>MAEYKDNLLGEANSFLEVLEQVSHLAPLDKPVLIIGERGTGKELIASRLHYLSSRWQGPFISLNCAALNENLLDSELFGHEAGAFTGAQKRHPGRFERADGGTLFLDELATAPMMVQEKLLRVIEYGELERVGGSQPLQVNVRLVCATNADLPAMVNEGTFRADLLDRLAFDVVQLPPLRERESDIMLMAEYFAIQMCREIKLPLFPGFTERARETLLNYRWPGNIRELKNVVERSVYRHGTSDYPLDDIIIDPFKRRP[6x];>MQGSVTEFLKPRLVDIEQVSSTHAKVTLEPLERGFGHTLGNALRRILLSSMPGCAVTEVEIDGVLHEYSTKEGVQEDILEILLNLKGLAVRVQGKDEVILTLNKSGIGPVTAADITHDGDVEIVKPQHVICHLTDENASISMRIKVQRGRGYVPASTRIHSEEDERPIGRLLVDACYSPVERIAYNVEAARVEQRTDLDKLVIEMETNGTIDPEEAIRRAATILAEQLEAFVDLRDVRQPEVKEEKPEFDPILLRPVDDLELTVRSANCLKAEAIHYIGDLVQRTEVELLKTPNLGKKSLTEIKDVLASRGLSLGMRLENWPPASIADE[2x];> MVYSYTEKKRIRKDFGKRPQVLDVPYLLSIQLDSFQKFIEQDPEGQYGLEAAFRSVFPIQSYSGNSELQYVSYRLGEPVFDVQECQIRGVTYSAPLRVKLRLVIYEREAPEGTVKDIKEQEVYMGEIPLMTDNGTFVINGTERVIVSQLHRSPGVFFDSDKGKTHSSGKVLYNARIIPYRGSWLDFEFDPKDNLFVRIDRRRKLPATIILRALNYTTEQILDLFFEKVIFEIRDNKLQMELVPERLRGETASFDIEANGKVYVEKGRRITARHIRQLEKDDVKLIEVPVEYIAGKVVAKDYIDESTGELICAANMELSLDLLAKLSQSGHKRIETLFTNDLDHGPYISETLRVDPTNDRLSALVEIYRMMRPGEPPTREAAESLFENLFFSEDRYDLSAVGRMKFNRSLLREEIEGSGILSKDDIIDVMKKLIDIRNGKGEVDDIDHLGNRRIRSVGEMAENQFRVGLVRVERAVKERLSLGDLDTLMPQDMINAKPISAAVKEFFGSSQLSQFMDQNNPLSEITHKRRISALGPGGLTRERAGFEVRDVHPTHYGRVCPIETPEGPNIGLINSLSVYAQTNEYGFLETPYRKVTDGVVTDEIHYLSAIEEGNYVIAQANSNLDEEGHFVEDLVTCRSKGESSLFSRDQVDYMDVSTQQVVSVGASLIPFLEHDDANRALMGANMQRQAVPTLRADKPLVGTGMERAVAVDSGVTAVAKRGGVVQYVDASRIVIKVNEDEMYPGEAGIDIYNLTKYTRSNQNTCINQMPCVSLGEPVERGDVLADGPSTDLGELALGQNMRVAFMPWNGYNFEDSILVSERVVQEDRFTTIHIQELACVSRDTKLGPEEITADIPNVGEAALSKLDESGIVYIGAEVTGGDILVGKVTPKGETQLTPEEKLLRAIFGEKASDVKDSSLRVPNGVSGTVIDVQVFTRDGVEKDKRALEIEEMQLKQAKKDLSEELQILEAGLFSRIRAVLVAGGVEAEKLDKLPRDRWLELGLTDEEKQNQLEQLAEQYDELKHEFEKKLEAKRRKITQGDDLAPGVLKIVKVYLAVKRRIQPGDKMAGRHGNKGVISKINPIEDMPYDENGTPVDIVLNPLGVPSRMNIGQILETHLGMAAKGIGDKINAMLKQQQEVAKLREFIQRAYDLGADVRQKVDLSTFSDEEVMRLAENLRKGMPIATPVFDGAKEAEIKELLKLGDLPTSGQIRLYDGRTGEQFERPVTVGYMYMLKLNHLVDDKMHARSTGSYSLVTQQPLGGKAQFGGQRFGEMEVWALEAYGAAYTLQEMLTVKSDDVNGRTKMYKNIVDGNHQMEPGMPESFNVLLKEIRSLGINIELED;> MKDLLKFLKAQTKTEEFDAIKIALASPDMIRSWSFGEVKKPETINYRTFKPERDGLFCARIFGPVKDYECLCGKYKRLKHRGVICEKCGVEVTQTKVRRERMGHIELASPTAHIWFLKSLPSRIGLLLDMPLRDIERVLYFESYVVIEGGMTNLERQQILTEEQYLDALEEFGDEFDAKMGAEAIQALLKSMDLEQECEQLREELNETNSETKRKKLTKRIKLLEAFVQSGNKPEWMILTVLPVLPPDLRPLVPLDGGRFATSDLNDLYRRVINRNNRLKRLLDLAAPDIIVRNEKRMLQEAVDALLDNGRRGRAITGSNKRPLKSLADMIKGKQGRFRQNLLGKRVDYSGRSVITVGPYLRLHQCGLPKKMALELFKPFIYGKLELRGLATTIKAAKKMVEREEAVVWDILDEVIREHPVLLNRAPTLHRLGIQAFEPVLIEGKAIQLHPLVCAAYNADFDGDQMAVHVPLTLEAQLEARALMMSTNNILSPANGEPIIVPSQDVVLGLYYMTRDCVNAKGEGMVLTGPKEAERLYRSGLASLHARVKVRITEYEKDANGELVAKTSLKDTTVGRAILWMIVPKGLPYSIVNQALGKKAISKMLNTCYRILGLKPTVIFADQIMYTGFAYAARSGASVGIDDMVIPEKKHEIISEAEAEVAEIQEQFQSGLVTAGERYNKVIDIWAAANDRVSKAMMDNLQTETVINRDGQEEKQVSFNSIYMMADSGARGSAAQIRQLAGMRGLMAKPDGSIIETPITANFREGLNVLQYFISTHGARKGLADTALKTANSGYLTRRLVDVAQDLVVTEDDCGTHEGIMMTPVIEGGDVKEPLRDRVLGRVTAEDVLKPGTADILVPRNTLLHEQWCDLLEENSVDAVKVRSVVSCDTDFGVCAHCYGRDLARGHIINKGEAIGVIAAQSIGEPGTQLTMRTFHIGGAASRAAAESSIQVKNKGSIKLSNVKSVVNSSGKLVITSRNTELKLIDEFGRTKESYKVPYGAVLAKGDGEQVAGGETVANWDPHTMPVITEVSGFVRFTDMIDGQTITRQTDELTGLSSLVVLDSAERTAGGKDLRPALKIVDAQGNDVLIPGTDMPAQYFLPGKAIVQLEDGVQISSGDTLARIPQESGGTKDITGGLPRVADLFEARRPKEPAILAEISGIVSFGKETKGKRRLVITPVDGSDPYEEMIPKWRQLNVFEGERVERGDVISDGPEAPHDILRLRGVHAVTRYIVNEVQDVYRLQGVKINDKHIEVIVRQMLRKATIVNAGSSDFLEGEQVEYSRVKIANRELEANGKVGATYSRDLLGITKASLATESFISAASFQETTRVLTEAAVAGKRDELRGLKENVIVGRLIPAGTGYAYHQDRMRRRAAGEAPAAPQVTAEDASASLAELLNAGLGGSDNE;> MARVTVQDAVEKIGNRFDLVLVAARRARQMQVGGKDPLVPEENDKTTVIALREIEEGLINNQILDVRERQEQQEQEAAELQAVTAIAEGRR;> MKQGLQLRLSLAMTPQLQQAIRLLQLSTLELQQELQQALESNPLLEQTDLHDEVEAKEVEDRESLDTVDALEQKEMPDELPLDASWDEIYTAGTPSGNGVDYQDDELPVYQGETTQTLQDYLMWQVELTPFTDTDRAIATSIVDAVDDTGYLTIQIEDIVDSIGDDEIGLEEVEAVLKRIQRFDPVGVAAKDLRDCLLIQLSQFAKETPWLEEARLIISDHLDLLANHDFRTLMRVTRLKEEVLKEAVNLIQSLDPRPGQSIQTSEPEYVIPDVLVRKVSGRWTVELNADSIPRLKINQQYAAMGNSARNDADGQFIRSNLQEARWLIKSLESRNDTLLRVSRCIVEQQQAFFEQGEEYMKPMVLADIAQAVEMHESTISRVTTQKYLHSPRGIFELKYFFSSHVNTEGGGEASSTAIRALVKKLIAAENPAKPLSDSKLTSMLSEQGIMVARRTVAKYRESLSIPPSNQRKQLV

Bacteria use sigma (σ) factors to recruit RNA polymerase (RNAP) to promoter regions of genes that need to be transcribed, with 60% bacteria containing at least one specialized σ factor, σ54, responsible for transcribing many stress response genes. The σ54-mediated transcription initiation requires specific AAA+ proteins (ATPases Associated with diverse cellular Activities) known as bacterial enhancer-binding proteins (bEBPs). DNA looping enables bEBP hexamers to engage and actively remodel the RNAP-σ54-DNA closed complex to convert it into an open complex. In this work we capture intermediate states of bEBPs in facilitating DNA opening and partial unfolding of σ54, and therefore link the ATPase activity to DNA opening and σ54 remodeling, which eventually lead to transcription activation.

To understand the structural basis and how DNA is stabilized in these complexes, we determined the structures of PspF1-275-RNAP-σ54-DNA containing mismatches between −11 and −8 [RPi(−11/−8)] and between −10 and −1 [RPi(−10/−1)]. Interestingly, DNA with a partially opened bubble between −11 and −8 did not support transcription, suggesting that this complex is unable to proceed further to an open complex. In the RPi(−11/−8), we observe multiple structural conformations, at varying degrees of tilt of PspF1-275 hexamer ring relative to RNAP-σ54 and varying degrees of RNAP clamp opening We also observe significant degrees of promoter DNA bending, demonstrating the wide degree of conformational flexibility in the complex. The DNA density downstream of −10 was generally poorly resolved, indicating that this region was highly flexible. However, one conformation has sufficiently high resolution to allow us to resolve the DNA. In these complexes, we observe a previously unreported interaction between PspF and σ54 RpoN domain. This interaction is only possible with the tilted ring conformation, suggesting this interaction contributes to the stabilization of this ring conformation in both RPi(−11/−8) and RPi(−10/−1), giving rise to the higher-resolution reconstruction of these conformations. Significantly, we observe the σ54 N terminus is further shifted along the PspF hexamer in RPi(−11/−8) and RPi(−10/−1) compared to that of RPi(−12/−11). This would thus support the mechanistic model in which we proposed that ATP hydrolysis and the conformational changes within the hexamer lead to translocation of the σ54 N terminus; and RPi(−11/−8) and RPi(−10/−1) are further along the transcription initiation pathway. Second, PspF1-275 hexamer ring tilts, as observed in RPi(−11/−8) and RPi(−10/−1) structures, altering interactions between PspF1-275 and DNA, which could contribute to or stabilize DNA melting.>[2x]MVVAGIDP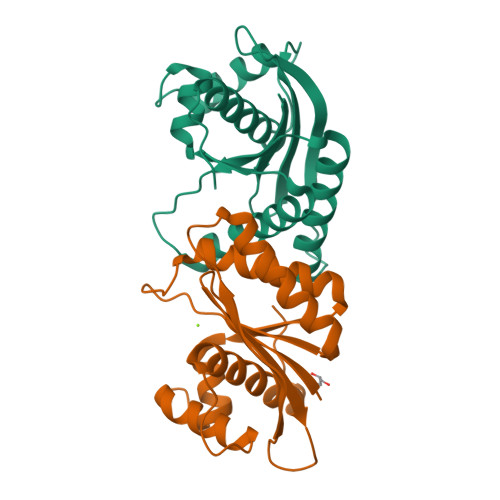GITHLGLGVVAVEGKGALKARLLHGEVVKTSPQEPAKERVGRIHARVLEVLHRFRPEAVAVEEQFFYRQNELAYKVGWALGAVLVAAFEAGVPVYAYGPMQVKQALAGHGHAAKEEVALMVRGILGLKEAPRPSHLADALAIALTHAFYARMGTAKPL>MTMITHHHHHHGSIVRRVDDIVWQSDYEYAIKHGNEYDYVISVAKECKHPRASLWIPQDDNVYIPADRYVTVYNFIKQHDNGKSKFLIHCCAGMSRSVAYSIAYLVLRYGITVSEA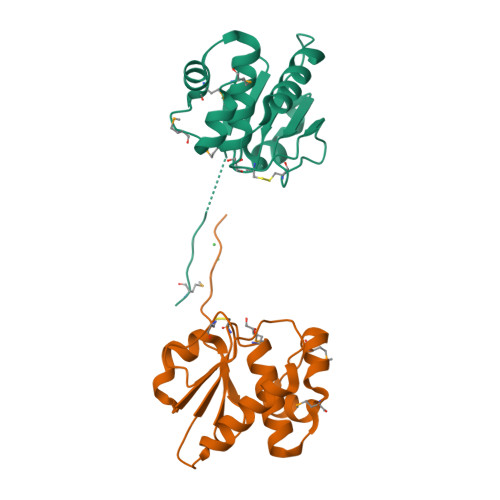KRRMGINYMLHPDIEKSLVM[2x]> MPTEFLYTSKIAAISWAATGGRQQRVYFQDLNGKIREAQRGGDNPWTGGSSQNVIGEAKLFSPLAAVTWKSAQGIQIRVYCVNKDNILSEFVYDGSKWITGQLGSVGVKVGSNSKLAALQWGGSESAPPNIRVYYQKSNGSGSSIHEYVWSGKWTAGASFGSTVPGTGIGATAIGPGRLRIYYQATDNKIREHCWDSNSWYVGGFSASASAGVSIAAISWG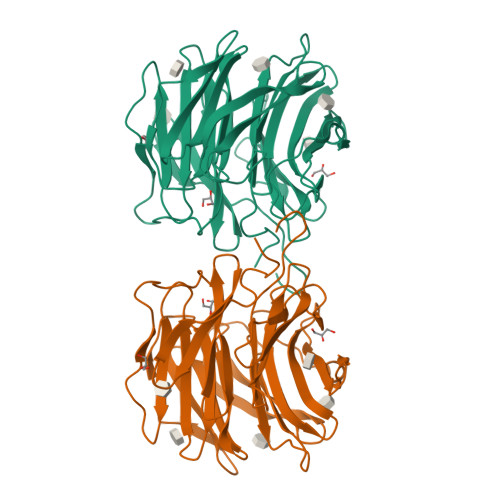STPQIRVYWQKGREELYEAAYGGSWNTPGQIKDASRPTPSLPDTFIAANSSGNIDISVFFQASGVSLQQWQWISGKGWSIGAVVPTGTPAGWLEHHHHHHHHHH> GPMSVPTDGAVTTSQIPASEQETLVRPKPLLLKLLKSVGAQKDTYTMKEVLFYLGQYIATKRLYDEKQQHIVYCSNDLLGDLFGVPSFSVK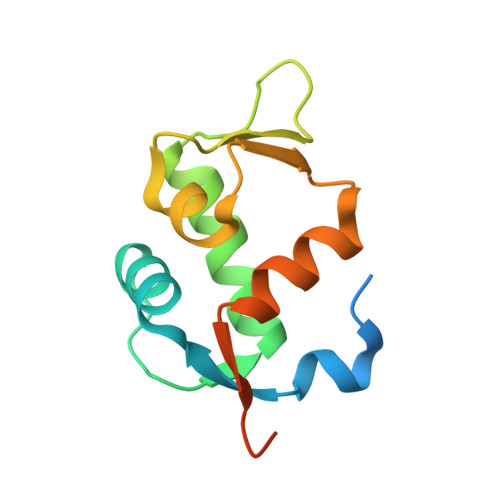EHRKIYTMIYRNLVVVNQQESSDSGTSVSEN>MDSTIRLVATIFLISLTQQIEVCNKAQQQGPYTLVDYQEKPLNISRIQIKVVKTS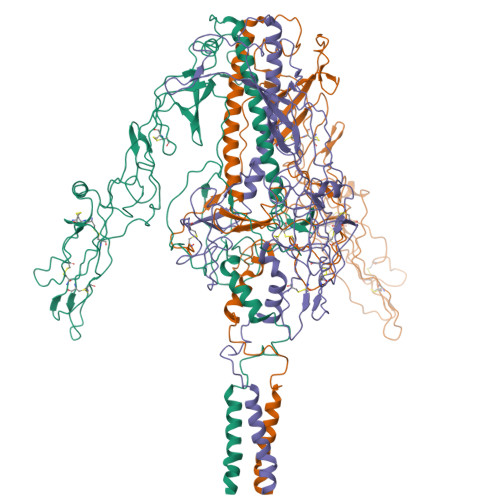VATKGLNFHIGYRAVWRSYCYNGGSLDKNTGCYNDLIPKSPTESELRTWSKSQKCCTGPDAVDAWGSDARICWAEWKMELCHTAKELKKYSNNNHFAYHTCNLSWRCGLKSTHIEVRLQASGGLVSMVAVMPNGTLIPIEGTRPTYWTEDSFAYLYDPAGTEKKTESTFLWCFKEHIRPTTELSGAVYDTHYLGGTYDKNPQFNYYCRDNGYYFELPANRLVCLPTSCYKREGAIVNTMHPDTWKVSEKLHSASQFDVNNVVHSLVYETEGLRLALSQLDHRFATLSRLFNRLTQSLAKIDDRLLGTLLGQDVSSKFISPTKFMLSPCLSTPEGDSNCHNHSIYRDGRWVHNSDPTQCFSLSKSQPVDLYSFKELWLPQLLDVNVEGVVADEEGWSFVAQSKQALIDTMTYTKNGGKGTSLEDVLGYPSGWINGKLQGLLLNGAISWVVVIGVVLVGVCLMRRVF[3x]In plants, flavonoid biosynthesis begins with phenylpropanoid metabolism in which phenylalanine is transformed into p-coumaroyl-coenzyme (Co)A. Chalcone synthase (EC 2.3.1.74), the first enzyme responsible for generating the basic flavonoid skeleton, then catalyzes the condensation of three molecules of malonyl-CoA with one molecule of p-coumaroyl-CoA to form chalcone. This is followed by the intramolecular and stereospecific cyclization of chalcone into (2S)-flavanone—a precursor of many downstream flavonoids—by chalcone-flavanone isomerase (CHI; EC 5.5.1.6). Type I CHIs—which are found in most plants including barley, rape, petunia, Arabidopsis, and rice—isomerize naringenin chalcone (2',4',6',4-tetrahydroxychalcone) into 5-hydroxy-flavonoid; whereas type II CHIs, common in leguminous plants, utilize both naringenin chalcone and isoliquiritigenin (2',4',4-trihydroxychalcone) to synthesize 5-deoxy-flavonoid. The family of genes encoding CHI in Deschampsia antartica—one of the only two vascular plant to naturally colonize the Maritime Antarctic—was recently characterized at the molecular level. The crystal structures of the unliganded and isoliquiritigenin-bound forms of DaCHI1 revealed that DaCHI1 can bind to type II substrates suggesting that DaCHI1 can produce antioxidant flavonoids from various substrates for protection against abiotic oxidative stresses.

Unliganded DaCHI1 was crystallized in the C2221 space group with two molecules in the asymmetric unit. Our analytical ultracentrifugation results showed that DaCHI1 is a monomer in solution with a standardized sedimentation coefficient of 2.14. The final model of the unliganded DaCHI1 structure contained 218 amino acid residues in a β-sandwich fold with seven α-helices (α1–α7) and seven β-strands (β1–β7). The β1 and β2 strands formed a short β-hairpin structure and β3–β7 strands formed an antiparallel β sheet. The seven α-helices were located at the concave surface of β-sheets and the active site was formed between the antiparallel β-sheet and α-helices. The substrate-binding cleft of DaCHI1 was conserved, with hydrophobic residues from β3 (Met36 and Ile38), β4 (Ile43, Phe45, and Ile48), β5 (Val94 and Met96), Leu100 of loop 97–101, α4 (Tyr105 and Val109), α6 (Ile190), and Val196 of loop 192–197. Several important catalytic residues including Arg34 (Arg36), Thr46 (Thr48), Tyr105 (Tyr106), Lys108 (Lys109), Asn112 (Asn113), and Ser189 (Thr190) were also preserved (residues in parentheses refer to those in MsCHI). The final model showed Rcryst and Rfree values of 0.222 and 0.278, respectively.

>[2x]MAVSELEVDGVVFPSLARPPGSAHSHFLAGAGVRGMEIGGNFIKFTAIGVYLQADAAVSALAKKWAGKAADELASDAAFFRDVVTGEFEKFTQVTMILPLTGAQYSEKVTENCVAYWKAVGAYTDAEAAAVDKFKEAFKTETFPPGASILFTHSPAGVLTVAFSKNSSVPESGGAAIENRPLCEAVLESIIGEHGVSPAAKLSLATRVAELLKEAASVDEPAAAEPVSVSA> MSENCNHIVTTLKRDGTGRRDLLDPKLAPESVQLQDFELSDWLIFALNFARKIHFFPSDLANEPLGDWRNFFSTIVSDKTLISDIENLDDFEKLRGNIEEFLAAYDQSGKLTPHLTLFVSFLKLLETSKKRFNQLTKRHLDFYYQEILHLEKQALSPDHVFLIFELAKNVSQEKLDEGTEVDGGKDDTGKKNTYLTSFETVLNKTKVGQLKSLYNEISVEKEEIKELNTPISTGTFVMAPMANSFDGLGEDFPKGSEKWWPFGYTKICNASTVLPALPKARLGCSISSKLLKLSEGTRDIILEFTFNKPILPNGEDYTALNKAMSIELTGEKGWIAGLPMTLKSDSGINSGSKKMKLSLTLDSEQPAVVPYQTELHEGSYEVDEPLLRVLFKTNEKEGYNLYRLFNENVLTDLKITVEVSDITSVQLENDLGVLNPQKPFFPFGPRPIKGSSFIVKYPEAMEKPVTAISYQMDYLNLPENLVNHYSAYTIGDDEPLVSDMDYFSVKSFPKSSNDSDQLFSEKSGGGYESDFEFQIENGVWESGLKKELKISLERSFLHEKYAHYFTLVAISKDTDPTIE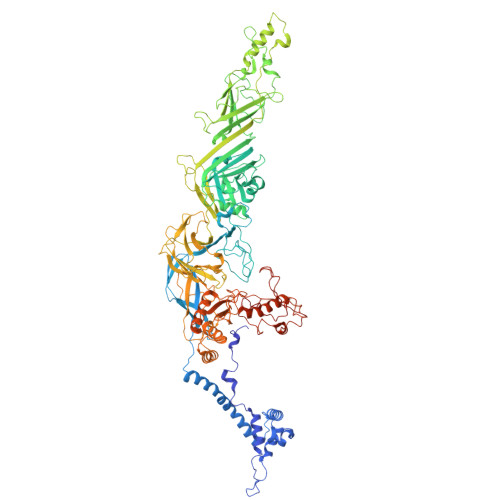LLPNEPYAPLAENLVLGYTAISSIDFSSSSSENQVSLIHEMPFGFQQVFTPGDTDNSLYLVPDYCHGGELYIGLENGKNLQQVTLLLQFLEGSENPDITDIFTGNQKIKWQYLSQNQWQDFQSGEIIQNQTPRFLKSGIFQFSIPKQANLDNTVLPPGYHWIKASMVKPFDVVSQLINIHAQAVEAVFEDQGSSGNHLEKGLPAETISKLQERLSWIKSIQQPYPSTKGKAQESDEDYYRRVSERLRHKKRAITLWDYEHLILQKFPKVYKVKCLNHTCSSSFQSPGNATLILVPDTVQQSVFDIYQPRVSQGTLNDVAAFVNELNSFHVQAKVINPNYEEVKVDVKVKFREGLDVSFYLTKVKEDIKKFLSPWAYDQESSVEFGVTLHRSQMIHYLEQLTYVDYITDLRLLKRQAGSSPCNPIFIETTEKEYIQPSNPKSILVSAKEHLVTPITQNCSSISLNNEEECQH>AECSVDIQGNDQ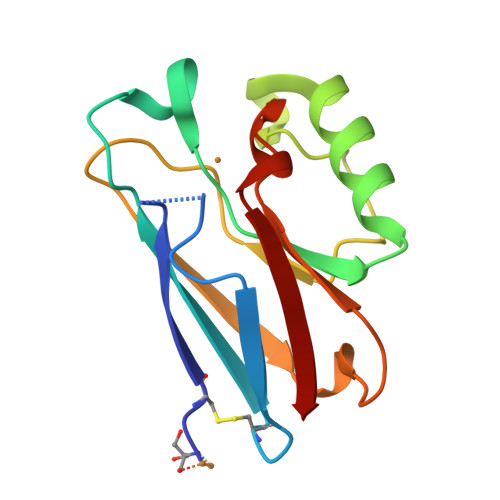MQFNTNAITVDKSCKQFTVNLSHPGNLPKNVKGHNWVLSTAADMQGVVTDGMASGLDKDYLKPDDSRVIAHTKLIGSGEKDSVTFDVSKLKEGEQYMFFCTFPGHSALEKGTLTLK[2x]>MSVVPPNRSQTGWPRGVTQFGNKYIQQTKPLTLERTINLYPLTNYTFGTKEPLYEKDSSVAARFQRMREEFDKIGMRRTVEGVLIVHEHRLPHVLLLQLGTTFFKLPGGELNPGEDEVEGLKRLMTEILGRQDGVLQDWVI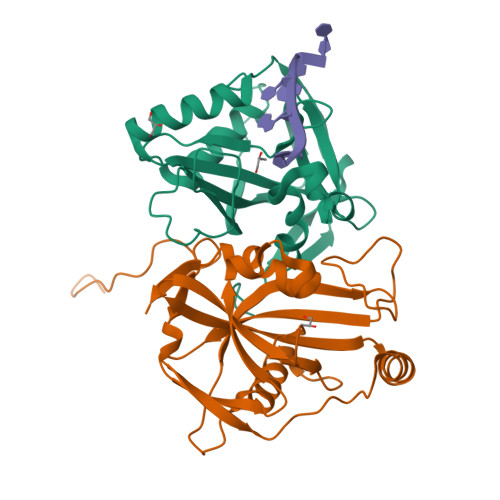DDCIGNWWRPNFEPPQYPYIPAHITKPKEHKKLFLVQLQEKALFAVPKNYKLVAAPLFELYDNAPGYGPIISSLPQLLSRFNFIYN[2x]Phosphoketolase (XPK) belongs to the transketolase family, a member of thiamine pyrophosphate (TPP)-dependent enzyme superfamily. It converts F6P, xylulose-5-phosphate (Xu5P) or sedoheptulose-7-phosphate (S7P), which are intermediates in RuBP regeneration, to produce acetyl phosphate (AcP) and C3, C4 or C5 sugar phosphates. XPK is an enzyme present in many microorganisms, primarily involved in substrate-level phosphorylation to produce AcP.

Given the importance of the physiological role of SeXPK, we solved the cryo-EM structures of SeXPK, both free (with coenzyme TPP/Mg2+ bound) and complexed with the non-hydrolyzable ATP analog, AMPPNP. In contrast to the published XPK structures from Lactococcus lactis and B. breve/longum, which exist as dimers in crystals, the cryo-EM structure of SeXPK is a dodecamer composed of six dimeric units, forming a circular donut-shaped array both for the AMPPNP-bound form and in the absence of AMPPNP. Using cryo-EM analysis, we discovered that these functions were enabled by a unique allosteric regulatory site involving two subunits jointly binding two ATP, which constantly suppresses the activity of SeXPK until the ATP level drops. Comparison between the free and bound dimers in the same orientation shows that the two subunits jointly bind two AMPPNP. The key residues, H706 and Y710 from reciprocal subunits (helix α24 based on Supplementary Fig. 3), sandwich AMPPNP in the dimer interface by forming π–π stacking interactions with the adenine ring of AMPPNP. The α- and β-phosphate groups of AMPPNP are stabilized by H706, H719, R721 and R753 and the γ-phosphate group by R711 from the reciprocal subunit. Of note, while the dimer–dimer interface in the SeXPK dodecamer involves residues near the C terminus, the B. longum XPK octamer involves residues near the N terminus. As the donut-shape or four-leaf clover shape-like particles or two-dimensional (2D) class average images were not in perfect symmetry, we further examined whether the assigned symmetries were pseudosymmetry. Some relative random motions were observed between different dimers in both SeXPK dodecamer and B. longum octamer assemblies, suggesting the likelihood of pseudosymmetry in these structures. The root-mean-square deviation between the structures with and without AMPPNP-bound is very small: (0.42 Å from 7,897 Cα atoms of the dodecamer and 0.36 Å from 1,256 Cα atoms of the dimer).

>[12x]MTSTLQATDIATLSPNEQAAIDAWWRAANYLSVGQIYLRDNPLLQEPLRPEHIKQRLLGHWGSDPGLSFVYVHLNRLIRRLDLNLIYVTGPGHGAPALLANAWLEGTYSEVYPNCQQSTAGLQQFFKQFSFPGGIGSHCTPETPGSIHEGGELGYSLSHAFGAALDNPDLIVACVIGDGEAETGPLATSWHSNKFLNPAQDGAVLPILHLNGYKIANPTLLSRISHEELRSLFIGYGYEPFFVEGNDPAILHGVMASTLATCVQKIQAIQAAARSGESSDRPMWPMIVLRTPKGWTGPATIKGHVVEGSWRSHQVPMADVLTNPEHLQLLEDWLRSYRPEELFDASGAPVAELQAIAPIGDRRMSANPVTNGGLLRRALTLPDFRDQAVSVPAPGKSRADSTRPLGQFLREVIRHNPDNFRLFGPDETASNRLDAVYEVTSKVWLGDRIPEDEDGGHLSDRGRVMEILSEHTLEGWLEAYLLTGRHGFFATYEAFAHVIDSMVNQHAKWLDVSKREVDWRAPVSSLNILLSSTVWRQDHNGFSHQDPGFIDLVTNKSARVTRIYLPPDANCLLSVADHCLRSTDYINVIVADKQSHLQYLDAEAAARHCAKGIGIWDWASNDQGASPDVVIASCGDVVTLEALAATALLREHFPDLKIRFVNVVDLFRLQPDTEHPHGLSDRDFDSLFTVDKPIIFNFHGYPWLIHKLAYRRHNHNNLHVRGYKEVGNINTPLELAIRNQVDRFNLAIDVIDRVPHLRDRGAHVKEWLKDQIHDHIQYAYQEGIDRPEINQWQWPF>MIFVKNLASVLSQEWSSTEKYPGVRWKFLIDADFDGSSGLSLGFAEIAPGGDLTLHYHSPAEIAVVTNGKGILNKSGKLETIKKGDVVYIAGNAEHALKNNGKETLEFYWIFPTDRFSEVEYFPAKQKSGHHHHHH[2x]

Dimethylsulfoxonium propionate (DMSOP) is a recently identified and abundant marine organosulfur compound with roles in oxidative stress protection, global carbon and sulfur cycling and, as shown here, potentially in osmotolerance. Microbial DMSOP cleavage yields dimethyl sulfoxide, a ubiquitous marine metabolite, and acrylate, but the enzymes responsible, and their environmental importance, were unknown. Here we report DMSOP cleavage mechanisms in diverse heterotrophic bacteria, fungi and phototrophic algae not previously known to have this activity, and highlight the unappreciated importance of this process in marine sediment environments. These diverse organisms, including Roseobacter, SAR11 bacteria and Emiliania huxleyi, utilized their dimethylsulfoniopropionate lyase ‘Ddd’ or ‘Alma’ enzymes to cleave DMSOP via similar catalytic mechanisms to those for dimethylsulfoniopropionate. Like dddY, cloned dddL, dddQ, dddW, dddK and dddU conferred DMSOP lyase activity even with equimolar DMSP present, which was not surprising considering the similar structures of DMSP and DMSOP, and that these DMSP lyases have cupin domains and similar catalytic mechanisms.

Residues His56, His58, Glu62, His96 and the DMSOP molecule coordinated the Mn2+. In addition to the coordination bond between Mn2+ and DMSOP, a hydrogen bond between Tyr122 and DMSOP helped locate the carboxyl group of DMSOP in the DddK active site, potentially explaining why the Tyr122 substitution reduced DMSOP lyase activity by >90%. The positively charged dimethylsulfoxonium moiety of DMSOP was located exactly where DMSP was in the DddK–DMSP complex and was stabilized via cation–π interactions to the side chains of several aromatic residues, including Tyr21, Trp26, Phe108, Trp110 and Phe117, which, except for Tyr21, also perfectly superposed onto the DddK–DMSP complex. The Tyr21 side chain moved ~1 Å away from DMSOP compared with that of DMSP, providing a wider substrate-binding pocket to accommodate the DMSOP dimethylsulfoxonium moiety, which is larger than the sulfonium of DMSP. Structural analysis also highlighted Tyr64 and Tyr122 as the probable DddK DMSOP cleavage catalytic residues, although the distance between the Tyr64 hydroxyl and the C-alpha of DMSOP was >4 Å. From these data, we proposed that the DddK catalytic mechanism for DMSOP mirrored that for DMSP29. When DMSOP binds to DddK, it displaces the water molecule and forms a new coordination bond with Mn2+. Subsequently, the catalytic residue Tyr64 attacks the Cα–H proton of DMSOP, forming a Cα carbanion. Then, the Cα carbanion attacks the Cβ of DMSOP, leading to the breaking of the Cβ–S bond. Consequently, DMSOP is cleaved into DMSO and acrylate, which is then released from the DddK active site.>[2x]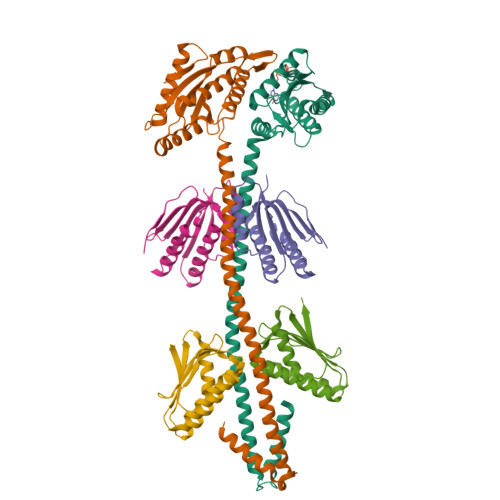SMSRERELDAWIDGLLADPQFHGHPLHQALARLRQQSLEQLVRLERIARISDGFQSMAREQNLSLSERYHKQLRRLEKVARISDRYQQMMRDLNLALKEASIRDPLTGLPNRRMLLERLREENERSQRHGQSYVLAMLDVDFFKQVNDTWGHDSGDRVLVEIARAMESELREYDLCGRWGGEEFLLLLPQTRLQDAGPVLERVRDSVRTLAVRVGTEALSVTASVGVTEHRIGETYSQTVNRADAALLDAKRSGRDKCVFAALPPLPAPSRPAPAR;>SMSDLHIPGTQSTPAIQGDWQAGRLSMQGDSYPENSYELFGQVIDWVERFLADGQRPLELDLRLLYLNTSSIKAMMDILDLLEEAHQGGRPVSLRWHYDRRNERVAELAEEFREDCSFPFAIQAHDE[4x]> GPHMLEAEHPLQYNYTFWYSRRTPGRPTSSQSYEQNIKQIGTFASVEQFWRFYSHMVRPGDLTGHSDFHLFKEGIKPMWEDDANKNGGKWIIRLRKGLASRCWENLILAMLGEQFMVGEEICGAVVSVRFQEDIISIWNKTASDQATTARIRDTLRRVLNLPPNTIMEY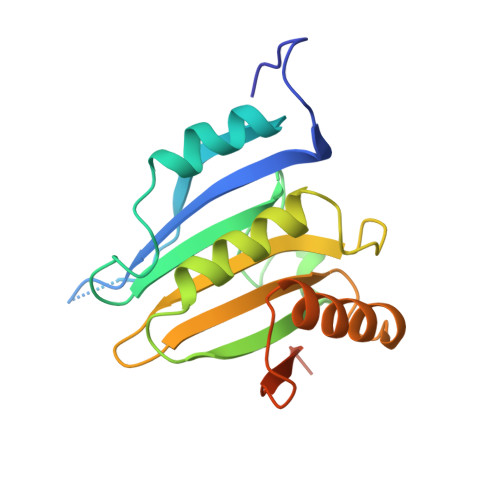KTHTDSIKMPGRLGPQRLLF> UCGUAACC;> CCCUCU;> GGUUUGGAGGGAAAAGUUAUCAGGCAUGCACCUGGUAGCUAGUCUUUAAACCAAUAGAUUGCAUCGGUUUAAAAGGCAAGACCGUCAAAUUGCGGGAAAGGGGUCAACAGCCGUUCAGUACCAAGUCUCAGGGGAAACUUUGAGAUGGCCUUGCAAAGGGUAUGGUAAUAAGCUGACGGACAUGGUCCUAACCACGCAGCCAAGUCCUAAGUCAACAGAUCUUCUGUUGAUAUGGAUGCAGUUCACAGACUAAAUGUCGGUCGGGGAAGAUGUAUUCUUCUCAUAAGAUAUAGUCGGACCUCUCCUUAAUGGGAGCUAGCGGAUGAAGUGAUGCAACACUGGAGCCGCUGGGAACUAAUUUGUAUGCGAAAGUAUAUUGAUUAGUUUUGGAGU

Group I introns catalyze their own excision from RNA precursors in many organisms through two sequential transesterification reactions. The Tetrahymena thermophila group I self-splicing intron was the first ribozyme to be discovered. To understand how the group I intron promotes catalysis and coordinates self-splicing reactions, we determine the structures of L-16 Tetrahymena ribozyme in complex with a 5′-splice site analog product and a 3′-splice site analog substrate using cryo-EM.

In Con1, the 5′-splice site analog product S1 forms six base pairs with the IGS at the 5′-end of the intron to form the helix P1, docking into the G-binding site. A301 and A302 from J8/7 continuously stack and make A-minor interactions with base pairs in P1; G303 also interacts with another base pair in P1. Such tertiary interactions are critical for positioning the P1 helix. In the G-binding site, G(−1)S2 forms a base triple with the G264-C311 base pair in P7, consistent with the guanosine-to-G·C base triple postulated in a previous study. In our structure, 5′UCG of the S2 mimics the intron’s 3′-terminus and interacts with G313 and A314 in P7 to form a 2-bp P9.0 duplex-like stem, P7 extension. It likely promotes substrate binding by anchoring the strand close to the G-binding site and stacking upon the A263-C262-G312 base triple. This hypothesis is supported by the fact that the P7 extension (P7ext) formation precedes P10 formation, as demonstrated by the partial binding of S2 to IGSext. Besides, the high-resolution cryo-EM map allows us to confidently build the 3-bp P9a stem, which cannot be unambiguously resolved in our previous structures. In contrast to the hydrogen bond formed between the 2′-OH group of C262 and the exocyclic amino (N2) group of guanosine substrate in all conformations, the 2′-OH of A261 forms a hydrogen bond with the N2 of guanosine substrate selectively. This hydrogen bond is not formed in Con1 but instead forms in Con2-4.> QFRVIGPGYPIRALVGDEAELPCRISPGKNATGMEVGWYRSPFSRVVHLYRNGKDQDAEQAPEYRGRTELLKETISEGKVTL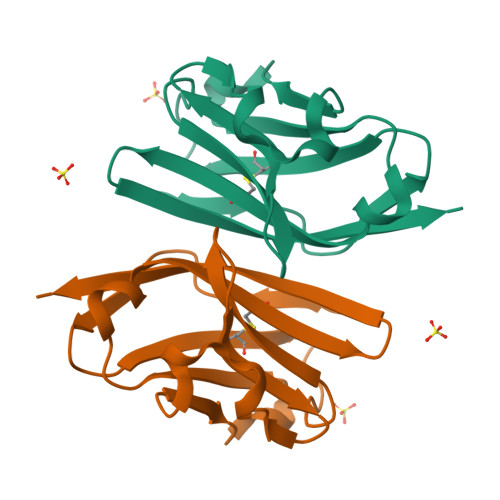RIQNVRFSDEGGYTCFFRDHSYQEEAAMELKVED>RSENITQWNLQDNGTEGIQRAMFQRGVNRSLHGIWPEKICTGVPSHLATDTELKAIHGMMDASEKTNYTCCRLQRHEWNKHGWCNWYNIEPWILLMNKTQANLTEGQPLRECAVTCRYDRDSDLNVVTQARDSPTPLTGCKKGKNFSFAGILVQGPCNFEIAVSDVL[2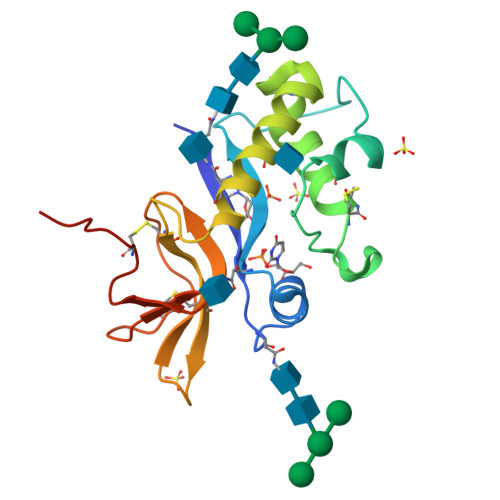x]> MGSSHHHHHHSQDPNSMPDNTIQWDKDADGIVTLTMDDPSGSTNVMNEAYIESMGKAVDRLVAEKDSITGVVVASAKKTFFAGGDVKTMIQARPEDAGDVFNTVETIKRQLRTLETLGKPVVAAINGAALGGGLEIALACHHRIA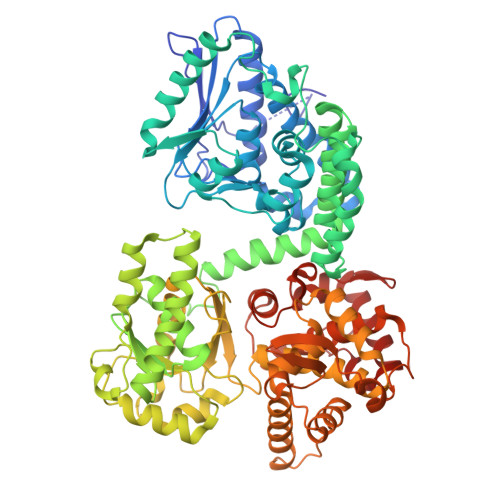ADVKGSQLGLPAVTLGLLPGGGGVTRTVRMFGIQNAFVSVLAQGTRFKPAKAKEIGLVDELVATVEELVPAAKAWIKEELKANPDGAGVQPWDKKGYKMPGGTPSSPGLAAILPSFPSNLRKQLKGAPMPAPRAILAAAVEGAQVDFDTASRIESRYFASLVTGQVAKNMMQAFFFDLQAINAGGSRPEGIGKTPIKRIGVLGAGMMGAGIAYVSAKAGYEVVLKDVSLEAAAKGKGYSEKLEAKALERGRTTQERSDALLARITPTADAADFKGVDFVIEAVFENQELKHKVFGEIEDIVEPNAILGSNTSTLPITGLATGVKRQEDFIGIAFFSPVDKMPLVEIIKGEKTSDEALARVFDYTLAIGKTPIVVNDSRGFFTSRVIGTFVNEALAMLGEGVEPASIEQAGSQAGYPAPPLQLSDELNLELMHKIAVATRKGVEDAGGTYQPHPAEAVVEKMIELGRSGRLKGAGFYEYADGKRSGLWPGLRETFKSGSSQPPLQDMIDRMLFAEALETQKCLDEGVLTSTADANIGSIMGIGFPPWTGGSAQFIVGYSGPAGTGKAAFVARARELAAAYGDRFLPPESLLS> MHHHHHHENLYFQGSGADKPSASNLIWSDEPAVVVYPQEDKNSEGSFGKYRKPASVWEAEGYPIGNGRVGAMIFSAPGRERLALNEISLWSGGANPGGGYGYGPDAGTNQFGNYLPFGDLFVDFKKGDQPASLSVEDFTRSLDLRDGIHKVNYKADGVTYDREAFSSTPANVLVLNYKASKPGQFSADFSVNSQLGADISAKGSVITWKGMLKNGMNYEGRVLIRPKGGTLSASGDKISVKNADSCMVVIAMETDYLMDYKKDWKGESPSRKLDRYAAKAASADYAALKQAHISQYKSMFDRVKVNFGKTEEDVAKLPTPKRLEAYKKNPADPDLEETMFQFGRYLLLSSSRPGTLPANLQGLWNDYVKPPWACDYHNNIN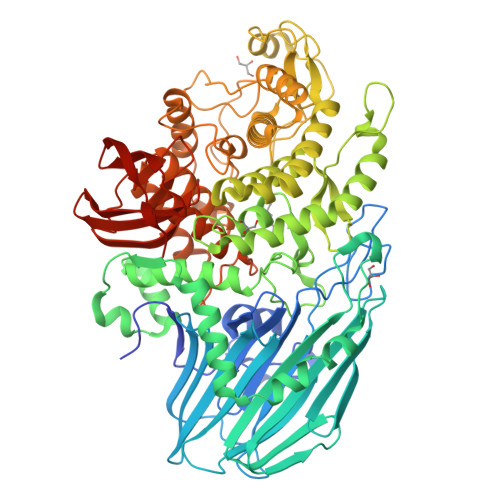VQMAYWGAEPANLSECHEALVNYVEAMAPGCRDASQANKGFNTKDGKPVRGWTVRTSQNIFGGNGWQWNIPGAAWYALHIWEHYAFTGDRKYLEKQAYPLMKEICHFWEDHLKELGAGGEGFKTNGKDPSEEEKKDLADVKAGTLVAPNGWSPAHGPREDGVMHDQQLIAELFSNTIKAARILGKDAAWAKSLEGKLKRLAGNKIGKEGNLQEWMIDRIPKTDHRHTSHLFAVFPGNQISKLKTPKLAEAARLSLEWRGTTGDSRRSWTWPWRTALWARLGEGNKAHEMVQGLLKFNTLPNMLTTHPPMQMDGNFGIVGGICEMLVQSHAGGLDIMPSPVEAWPEGSVKGLKARGNVTVDFSWKDGKVSNVKLYSAQPKVLPVRVNGKMTRMKTLPLKSGAGSSQPAAR> EEDLNWWEQENLRIAMKGERRWETLAHNGVLFPPEYEPHGIPIFYDGREFKMTPEEEEVATMFAVMKEHDYYRMEVFRRNFFESWREILDKRQHPIRRLELCDFEPIYQWHLVQREKKLSRTKEEKKAIKEKQDAEAEPYRYCVWDGRREQVANFRVEPPGLFRGRGKHPLMGKLKVRVQPEDITINIGETAEVPVPPAGHKWAAVQHDHTVTWLAMWRDSVAGNMKYVMLAPSSSVKGQSDMVKFEKARKLKDKVDDIRASYMEDFKSNDLHVAQRAVAMYFIDRLALRVGNEKGEDEADTVGCCSLRVEHIQLMPDNIVRFDFLGKDSIRYQNDVAVLPEVYALLQRFTRRKSPGMDIFDQLNPTQLNDHLKSFMDGLSAKVFRTYNASITLDRWFKEKPVDPKWSTADKLAYFNKANTEVAILCN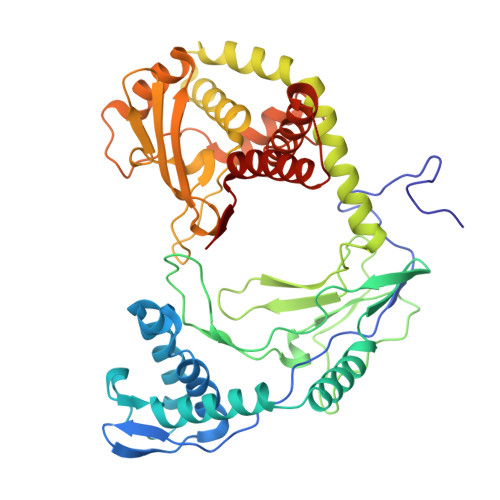HQKS Here, we have functionally and structurally characterized a representative of the PR family found in a widely distributed clade of marine actinobacteria, Candidatus Actinomarina minuta, named MAR [marine actinobacterial rhodopsin or MacR (16)]. In summary, the sequence alignment and the photocycle measurements confirm that MAR is a member of the PR family, which functions as an outward proton pump at neutral and high pH. Overall, MAR consists of seven transmembrane helices, A to G, connected through short intracellular and extracellular loops. A retinal chromophore is covalently bound to Lys200 of helix G. The fold of the MAR is similar to that of other PRs.

The orange-form crystals that were used to solve the MAR ground state structure under proton-pumping conditions also grew at pH 5.2, i.e., under pumping-inhibited conditions. We determined a 1.6-Å-resolution structure from such crystals, which provided a molecular basis for the inhibition of proton pumping in PRs under acidic conditions and the role of the His-Asp pair in it. In contrast, the structure of MAR under pumping-inhibited conditions shows that His51 and Asp72 reorient to form a 2.5-Å short H-bond (SHB). This reorientation of the residues and formation of an SHB indicate that this pair acquired a proton from the acidic solution. Reorientation of Asp72 toward His51 in the low-pH MAR leads to dehydration of the RSB region in a similar way to that shown for HsBR in the L and M states: Only one water molecule, w1*, remains in the region. Given the similarity between the structures of the M state and the acid blue (low pH) form of HsBR, the structure of MAR at low pH can be a reasonable model for the M state in the extracellular part of the pump. Considering these rationales, we will refer from here on to the structure of the orange-form MAR at high pH as the ground state and that at low pH as the M-like state. In contrast, under acidic conditions, the already protonated His-Asp pair cannot accept a proton from RSB, preventing RSB deprotonation and leading to the absence of the M state and proton pumping. While Arg82 of HsBR flips to the extracellular part in the acid blue and M states, Arg69 of MAR in the M-like state remains oriented toward RSB. It acquires some mobility, which is evident from the coexistence of two conformations.

>[2x]MEELTYRLFMVATVGMLAGTVFLLASSREVKPEHRRGVYISALVCGIAWYHYQKMGASWESGSYDTGLRYVDWVLTVPLMFVEVLAVTRKGAAYNEAVRNWGIAATVMIGAGYYGETSAAGSNEYWTGFVIAMATYVWLMRNLQAEGEGLKGDQAVAFENIKNLILVGWIIYPLGYIAPVVGDFDAIREVLYTIADIINKVGLGVLVLQMARVQSGEKVS> MRLLNRHSFVVKRKVSEDGHYNEDGDWVAS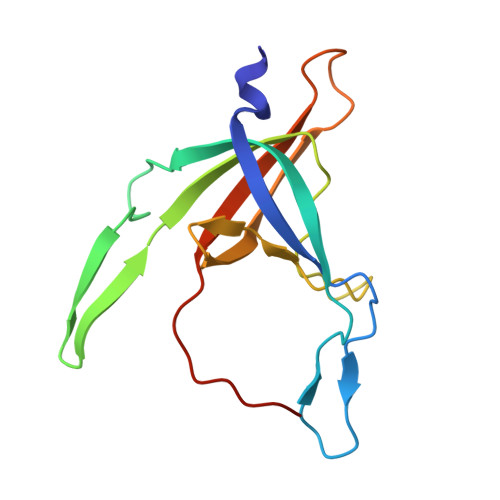QDVVSINCKGNIQPYIKGSVKNGTQIVLPEGIRLTDTRILFTVAELRTSDDVDWTEADIVMIKGHEYEVFMTMDWSEQLAHTSHYEYIIIRRDKMNAVRNSRT>KLKIEDFELHKMLGKGSFGKVFLAEFKKTNQFFAIKALKKDVVLMDDDVECTMVEKRVLSLAWEHPFLTHMFCTFQTKENLFFVMEYLNGGDLMYHIQSCHKFDLSRATFYAAEIILGLQFLHSKGIVYRDLKLDNILLDKDGHIKIADFGMCKENMLGDAKTNEFCGTPDYIAPEILLGQKYNHSVDWWSFGVLLYEMLIGQSPFHGQDEEELFHSIRMDNP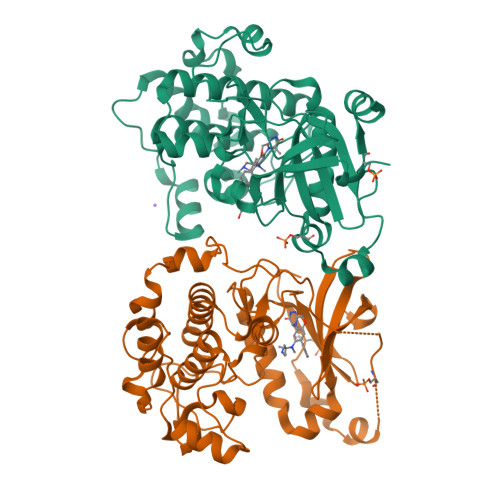FYPRWLEKEAKDLLVKLFVREPEKRLGVRGDIRQHPLFREINWEELERKEIDPPFRPKVKSPFDCSNFDKEFLNEKPRLSFADRALINSMDQNMFRNFSFMNPGMERLISH[2x]>[2x]MGSSHHHHHHSSGENLYFQGHMAAPFDKSRNVAQSIDQLIGQTPALYLNKLNNTKAKVVLKMECENPMASVKDRLGFAIYDKAEKEGKLIPGKS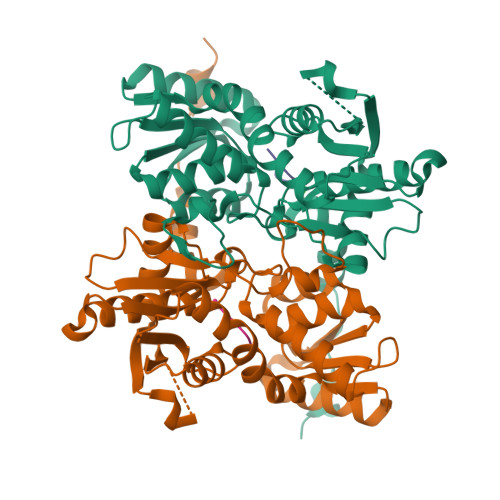VVVESSSGNTGVSLAHLGAIRGYKVIITMPESMSLERRCLLRIFGAEVILTPAALGMKGAVTMAKKIVTANPNAVLADQFATKYNALIHEETTGPEIWEQTNHNVDCFIAGVGTGGTLTGVARALKKMGSHARIVAVEPMESPVLSGGKPGAHKIQGIGPGFVPDVLDRSLIDEVFCVAGDDAIETALKLTRSDGVFCGFSGGANVYAALKIAERPEMEGKTIVTIIPSFGERYLSTALYRSVRDEVSSLPVVDASELQD;> EEEEE;> EEEE(2S,3S,5S)-5-[(N-FORMYL-L-LEUCYL)OXY]-2-HEXYL-3-HYDROXYHEXADECANOIC ACID | C29 H55 N O6 | 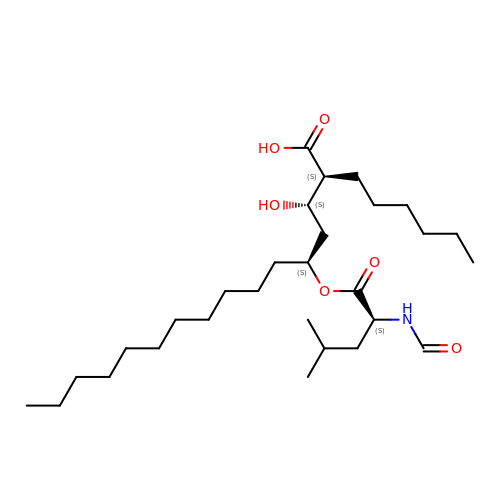FKUNIADJSAJLGB-FWEHEUNISA-N biphenyl-4-carboxylic acid 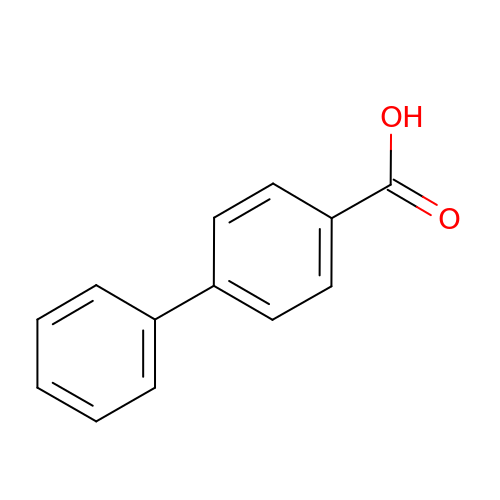| C13 H10 O2 | NNJMFJSKMRYHSR-UHFFFAOYSA-N> MNANLFARLFDKLDDPHKLAIETAAGDKISYAELVARAGRVANVLVARGLQVGDRVAAQTEKSVE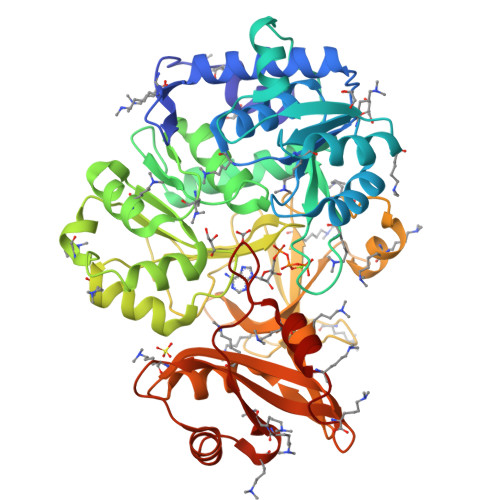ALVLYLATVRAGGVYLPLNTAYTLHELDYFITDAEPKIVVCDPSKRDGIAAIAAKVGATVETLGPDGRGSLTDAAAGASEAFATIDRGADDLAAILYTSGTTGRSKGAMLSHDNLASNSLTLVDYWRFTPDDVLIHALPIYHTHGLFVASNVTLFARGSMIFLPKFDPDKILDLMARATVLMGVPTFYTRLLQSPRLTKETTGHMRLFISGSAPLLADTHREWSAKTGHAVLERYGMTETNMNTSNPYDGDRVPGAVGPALPGVSARVTDPETGKELPRGDIGMIEVKGPNVFKGYWRMPEKTKSEFRDDGFFITGDLGKIDERGYVHILGRGKDLVITGGFNVYPKEIESEIDAMPGVVESAVIGVPHADFGEGVTAFVVLKREFAPSEAQVLHGLDGQLAKFKMPKKVIFVDDLPRNTMGAVQKNVLRETYKDIYK The cellular role of DNPH1 is to remove hydroxymethyl deoxyuridine monophosphate (hmdUMP) from the nucleotide pool. Hydrolysis generates deoxyribose monophosphate (dRP) and hydroxymethyl uracil (hmU) products. Glycosidic bond cleavage is driven by a conserved catalytic triad and proceeds via a two-step mechanism involving formation and subsequent disruption of a covalent glycosyl-enzyme intermediate. Each DNPH1 monomer adopts a Rossmann-like fold consisting of five core β-strands surrounded by five major α-helices.

In the first, an inactivating E104Q mutation permits binding of the intact substrate without cleavage. The purified protein (referred to as DNPH1E104Q) was co-crystallised with hmdUMP at 4 °C and X-ray diffraction data were collected from a single crystal. The six protein chains found in the asymmetric unit present as two full biologically active homodimers and two half homodimers; corresponding partners to the latter are defined by crystallographic symmetry. All copies are bound to substrate and are remarkably similar to each other (RMSD between Cα atom pairs = 0.128–0.406 Å), although there is some disorder for amino acids ~60–70, which form a loop across the top of the active site binding pocket. The core catalytic triad, consisting of Y24, D80 and E104Q, sits below the plane of the substrate deoxyribose sugar, poised for nucleophilic attack at the anomeric carbon. The base, which is held in plane by hydrophobic interactions from I29 and I76 side chains, adopts an anti conformation, with chi torsion angles (defined by O4′-C1′-N1-C2) of −178.9°, or 174.5 to 179.6°. The phosphate group is strongly coordinated by S98 and S128′, the latter being donated by the helical extension (amino acids 128′–133′) from the adjacent subunit. The same extension additionally positions the substrate hydroxymethyl group through a backbone amide interaction. At the other end of the substrate, the inactivating E104Q mutation introduces an amine group that forms an additional hydrogen bond with D80, pulling both catalytic residues away from the sugar. An additional interaction is observed between a base carbonyl oxygen (O2) and the sidechain of H56, which sits on the helical element immediately upstream of the shielding loop.

>[6x]GSMGRPALYFCGSIRGGREDRTLYERIVSRLRRFGTVLTEHVAAAELGARGEEAAGGDRLIHEQDLEWLQQADVVVAEVTQPSLGVGYQLGRAVAFNKRILCLFRPQSGRVLSAMIRGAADGSRFQVWDYEEGEVEALLDRYFEADP>[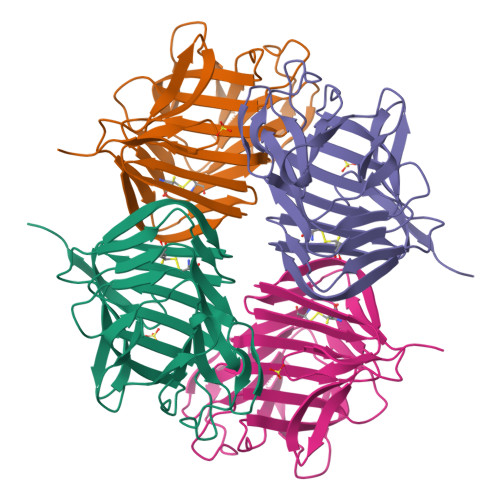2x]NGIVPDAGHQGPDVSAVNGGTQVINIVTPNNEGISHNQYQDFNVGKPGAVFNNALEAGQSQLAGHLNANSNLNGQAASLILNEVVSRNPSFLLGQAEVFGIAAEAVLSNPNGITCDGCGFINTSRSSLVVGNPLFENGQLKGYSTLNNTNLLSLGKNGLNTTGLLDLIAPRIDSRGKITAAEISAFTGQNTFSQHFDILSSQKPV>[8x]MEGPAGYLRRASVAQLTQELGTAFFQQQQLPAAMADTFLEHLCLLDIDSEPVAARSTSIIATIGPASRSVERLKEMIKAGMNIARLNFSHGSHEYHAESIANVREAVESFAGSPLSYRPVAIALDTKGPEIRTGILQGGPESEVELVKGSQVLVTVDPAFRTRGNANTVWVDYPNIVRVVPVGGRIYIDDGLISLVVQKIGPEGLVTQVENGGVLGSRKGVNLPGAQVDLPGLSEQDVRDLRFGVEHGVDIVFASFVRKASDVAAVRAALGPEGHGIKIISKIENHEGVKRFDEILEVSDGI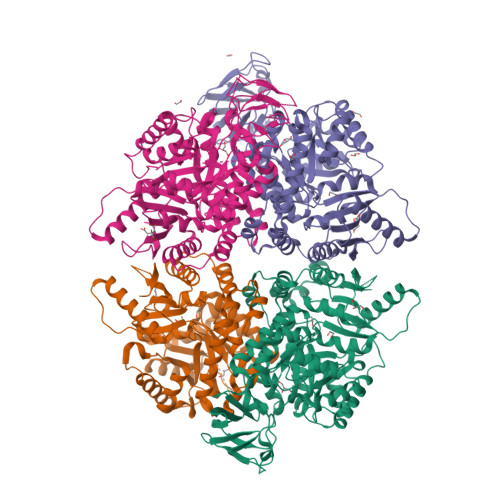MVARGDLGIEIPAEKVFLAQKMMIGRCNLAGKPVVCATQMLESMITKPRPTRAETSDVANAVLDGADCIMLSGETAKGNFPVEAVKMQHAIAREAEAAVYHRQLFEELRRAAPLSRDPTEVTAIGAVEAAFKCCAAAIIVLTTTGRSAQLLSRYRPRAAVIAVTRSAQAARQVHLCRGVFPLLYREPPEAIWADDVDRRVQFGIESGKLRGFLRVGDLVIVVTGWRGGGYTNIMRVLSIS> GPLGSKRQWTLEDFDIGRPLGKGKFGNVYLARERQSKFILALKVLFKTQLEKAGVEHQLRREVEIQSHLRHPNILRLYGYFHDATRVYLILEYAPLGTVYRE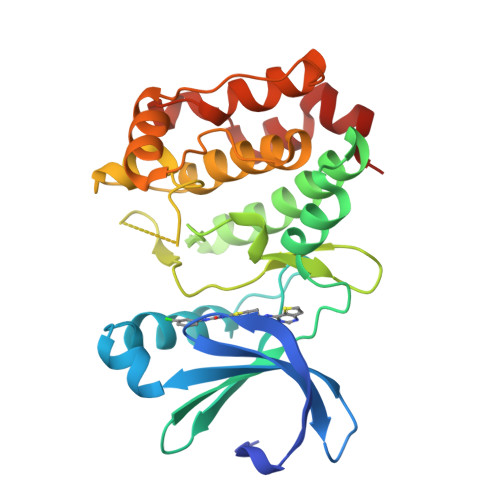LQKLSRFDEQRTATYITELANALSYCHSKRVIHRDIKPENLLLGSNGELKIADFGWSVHAPSSRRTTLCGTLDYLPPEMIEGRMHDEKVDLWSLGVLCYEFLVGMPPFEAHTYQETYRRISRVEFTFPDFVTEGARDLISRLLKHNASQRLTLAEVLEHPWIKANSSKPS>MYHSIKRFLIGKPLKSQAAGEQKLTKLKALAMLSSDALSSVAYGTEQILIILATISAAAFWYSIPIAVGVLILLLALILSYRQIIYAYPQGGGAYIVSKENLGEKPGLIAGGSLLVDYILTVAVSISAGTDAITSAFPALHDYHVPIAIFLVLVIMILNLRGLSESASILAYPVYLFVVALLVLIAVGLFKLMTGQIDQPAHHTSLGTPVAGITLFLLLKAFSSGCSALTGVEAISNAIPAFKNPPARNAARTLAMMGILLAILFSGITVLAYGYGTAPKPDETVVSQIASETFGRNVFYYVIQGVTSLILVLAANTGFSAFPQLAFNLARDQYMPRMFTVRGDRLGFSNGIIFLGFASIVLIILFGGQTEHLIPLYAVGVFIPFTLSQTGMCMKWIKQKPKGWIGKMLINSCGALISFMVLSILFVTKFNVVWPVLIFMPIVVLLFFAIKNHYTAVGEQLRIVDKEPEEIKGTVVIVPVAGVTTVVQKSIHYAKSLSDQVIAVHVSFDREQEKKFEKRWEELNNGVRLVTLHSSYRSLVHPFDKFLETVEAKAKKEQFSVMVLFPQF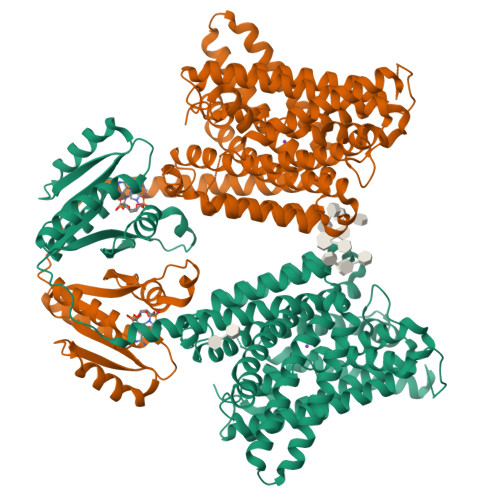ITKKRWHTILHNQSAFLLRVRLFWKKDIMVATLPYHFKK[2x]> MRSTQEERFEQRIAQETAIEPQDWMPDAYRKTLIRQIGQHAHSEIVGMLPEGNWITRAPTLRRKAILLAKVQDEAGHGLYLYSAAETLGCAREDIYQKMLDGRMKYSSIFNYPTLSWADIGVIGWLVDGAAIVNQVALCRTSYGPYARAMVKICKEESFHQRQGFEACMALAQGSEAQKQMLQDAINRFWWPALMMFGPNDDNSPNSARSLTWKIKRFTNDELRQRFVDNTVPQVEMLGMTVPDPDLHFDTESGHYRFGEIDWQEFNEVINGRGI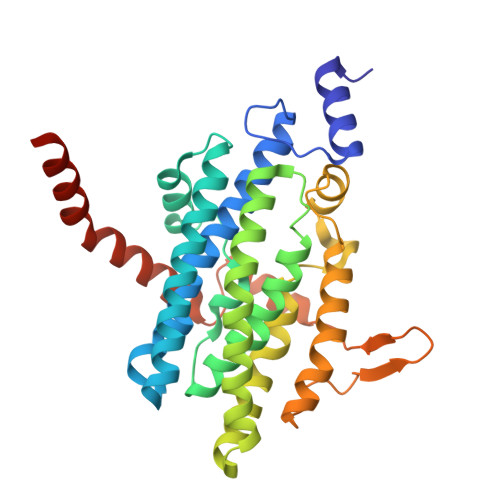CNQERLDAKRKAWEEGTWVREAALAHAQKQHARKVA> PIETVPVKLKPGMDGPKVKQWPLTEEKIKALVEICTEMEKEGKISKIGPENPYNTPVFAIKKKDSTKWRKLVDFRELNKRTQDFWEVQLGIPHPAGLKKKKSVTVLDVGDAYFSVPLDEDFRKYTAFTIPSINNKTPGIRYQYNVLPQGWKGSPAIFQSSMTKILEPFRKQNPDIVIYQYMDDLYVGSDLEIGQHRTKIEELRQHLLRWGLTTPDKKHQKEPPFLWMGYELHPDKWTVQPIVLPEKDSWTVNDIQKLVGKLNWASQIYPGIKVRQLCKLLRG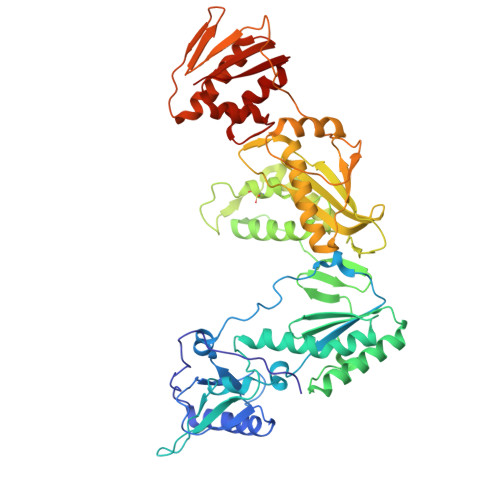TKALTEVIPLTEEAELELAENREILKEPVHGVYYDPSKDLIAEIQKQGQGQWTYQIYQEPFKNLKTGKYARMRGAHTNDVKQLTEAVQKITTESIVIWGKTPKFKLPIQKETWETWWTEYWQATWIPEWEFVNTPPLVKLWYQLEKEPIVGAETFYVDGAANRETKLGKAGYVTNRGRQKVVTLTDTTNQKTELQAIYLALQDSGLEVNIVTDSQYALGIIQAQPDQSESELVNQIIEQLIKKEKVYLAWVP1',5'-ANHYDRO-2',3'-DIDEOXY-2'-(5-IODOURACIL-1-YL)-D-ABABINO-HEXITOL 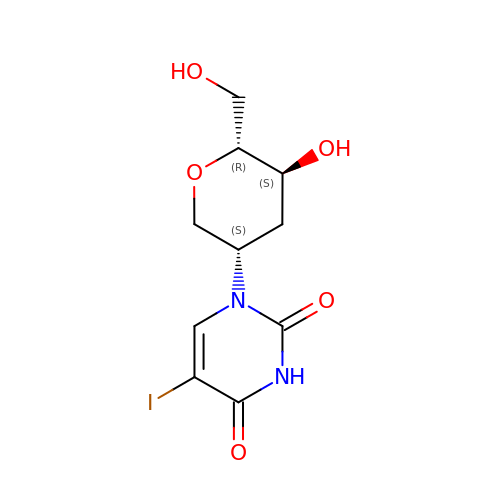| C10 H13 I N2 O5 | PJDQVZSBWDEYOF-APQOSEDMSA-N> MGFKGVGTYEIVPYQAPS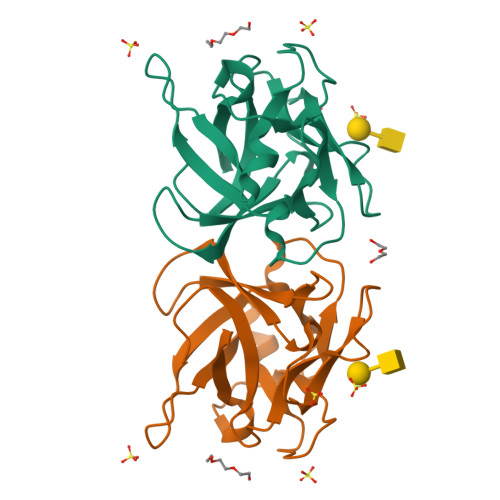LNLNAWEGKLEPGAVVRTYTRGDKPSDNAKWQVALVAGSGDSAEYLIINVHSGYFLTATKENHIVSTPQISPTDPSARWTIKPATTHQYEVFTINNKVSELGQLTVKDYSTHSGADVLSASAKTADNQKWYFDAK>MRGSHHHHHHGSMPVAGSELPRRPLPPAAQERDAEPRPPHGELQYLGQIQHILRCGVRKDDRTGTGTLSVFGMRARYSLRDEFPLLTTKRVFWKGVLEELLWFIKGSTNAKELSSKGVKIWDANGSRDFLDSLGFSTREEGDLGPVYGFQWRHFGAEYRDMESDYSGQGVDQLQRVIDTIKTNPDDRRIIMCAWNPRDLPLMALPPCHALCQFYVVNSELSCQLYQRSGDMGLGVPFNIASYALLTYMIAHITGLKPGDFIHTLGDAHIYLNHIEPLKIQLQREPRPFPKLRILRKVEKIDDFKAEDFQIEGYNPHPTIKMEMAV[8x]

Thymidylate synthase (TS, EC 2.1.1.45) plays a pivotal role in human cells, since it catalyzes the reductive methylation of 2′-deoxyuridine-5′-monophosphate (dUMP) to 2′-deoxythymidyne-5′-monophosphate (dTMP), using N5,N10-methylenetetrahydrofolate (mTHF) as cofactor. In human cells, TS provides the only synthetic source of dTMP necessary for DNA biosynthesis, indeed its inhibition halts the replication processes and induces apoptosis in rapidly dividing cells, an effect known as “thymineless death”. Former structural studies have revealed that the hTS homodimers are able to switch between two alternate conformations, named active and inactive, primarily by changing the orientation of the loop including the catalytic Cys195 (catalytic loop, residues 181–197). Human thymidylate synthase works as an obligate dimer, showing a stable quaternary assembly due to an extended inter-subunit interface.

The hTS variant Q62R, having the interface residue Gln62 replaced by arginine, was generated and characterized through kinetic assay, circular dichroism (CD) thermal denaturation analysis and X-ray crystallography. The structure of HT-hTS Q62R was solved to 2.55 Å resolution, showing that the mutated protein retains the constitutive dimeric quaternary structure of the wild-type enzyme. Four enzyme homodimers (A–B, C–D, E–F, G–H, in our model) were found in the cell asymmetric unit (ASU), all fully traced apart for the first twenty-five N-terminal residues (further the twelve residues belonging to the non-removable His6-tag). From the initial phases of structure solution and refinement, it was evident that HT-hTS Q62R was in the active conformation. Nonetheless, the analysis of the electron density in the active site area evidenced that the catalytic Cys195 was modified as S,S-(2-hydroxyethyl)thiocysteine (CME195) by the reaction with β-mercaptoethanol, added to the protein sample prior to the crystallization experiments. In all subunits, a sulfate anion was observed nearby the catalytic cysteine, anchored to the guanidinium moieties of the four arginine residues Arg50, Arg215, Arg175′, and Arg176’ (the last two from the partner subunit). Furthermore, in all active sites, the presence of a folate-like molecule was systematically observed. The active conformation adopted in the crystal by HT-hTS Q62R can be ascribed to the population of the cofactor site by 5-FTHF (the formation of the analogous complex in the wild-type enzyme has never been reported). However, the comparison of the mutant crystal structure with that of the wild-type enzyme in the active conformation suggests a likely explanation for the observed HT-hTS Q62R destabilization occurring in solution. The superimposition, displayed in Figure 6, provides clear evidence that the point-mutation Q62R induces a slight aperture of the enzyme dimer which is particularly visible in the area surrounding Arg62 and Arg62′ on the two enzyme halves.> MNESVKEIPDVLKSQCGFNCLTDISHSSFNEFRQQVSEHLSWSETHDLYHDAQQAQKDNRLYEARILKRANPQLQNAVHLAILAPNAELIGYNNQFSGRASQYVAPGTVSSMFSPAAYLTELYREARNLHASDSVYYLDTRRPDLKSMALSQQNMDIELSTLSLSNELLLESIKTESKLENYTKVMEMLSTFRPSGATPYHDAYENVREVIQLQDPGLEQLNASPAIAGLMHQASLLGINASISPELFNILTEEITEGNAEELYKKNFGNIEPASLAMPEYLKRYYNLSDEELSQFIGKASNFGQQEYSNNQLITPVVNSSDGTVKVYRITREYTTNAYQMDVELFPFGGENYRLDYKFKNFYNASYLSIKLNDKRELVRTEGAPQVNIEYSANITLNTADISQPFEIGLTRVLPSGSWAYAAAKFTVEEYNQYSFLLKLNKAIRLSRATELSPTILEGIVRSVNLQLDINTDVLGKVFLTKYYMQRYAIHAETALILCNAPISQRSYDNQPSQFDRLFNTPLLN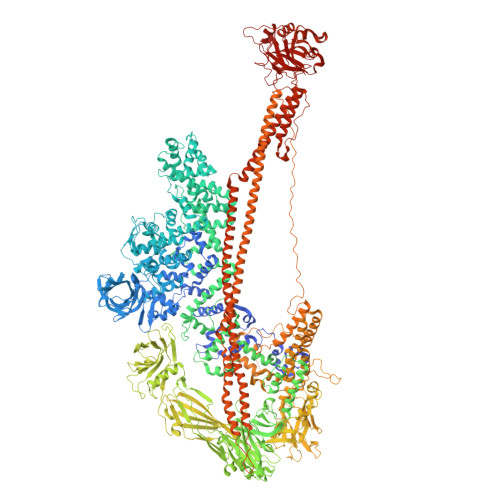GQYFSTGDEEIDLNSGSTGDWRKTILKRAFNIDDVSLFRLLKITDHDNKDGKIKNNLKNLSNLYIGKLLADIHQLTIDELDLLLIAVGEGKTNLSAISDKQLATLIRKLNTITSWLHTQKWSVFQLFIMTSTSYNKTLTPEIKNLLDTVYHGLQGFDKDKADLLHVMAPYIAATLQLSSENVAHSVLLWADKLQPGDGAMTAEKFWDWLNTKYTPGSSEAVETQEHIVQYCQALAQLEMVYHSTGINENAFRLFVTKPEMFGAATGAAPAHDALSLIMLTRFADWVNALGEKASSVLAAFEANSLTAEQLADAMNLDANLLLQASIQAQNHQHLPPVTPENAFSCWTSINTILQWVNVAQQLNVAPQGVSALVGLDYIQSMKETPTYAQWENAAGVLTAGLNSQQANTLHAFLDESRSAALSTYYIRQVAKAAAAIKSRDDLYQYLLIDNQVSAAIKTTRIAEAIASIQLYVNRALENVEENANSGVISRQFFIDWDKYNKRYSTWAGVSQLVYYPENYIDPTMRIGQTKMMDALLQSVSQSQLNADTVEDAFMSYLTSFEQVANLKVISAYHDNINNDQGLTYFIGLSETDAGEYYWRSVDHSKFNDGKFAANAWSEWHKIDCPINPYKSTIRPVIYKSRLYLLWLEQKEITKQTGNSKDGYQTETDYRYELKLAHIRYDGTWNTPITFDVNKKISELKLEKNRAPGLYCAGYQGEDTLLVMFYNQQDTLDSYKNASMQGLYIFADMASKDMTPEQSNVYRDNSYQQFDTNNVRRVNNRYAEDYEIPSSVSSRKDYGWGDYYLSMVYNGDIPTINYKAASSDLKIYISPKLRIIHNGYEGQKRNQCNLMNKYGKLGDKFIVYTSLGVNPNNSSNKLMFYPVYQYSGNTSGLNQGRLLFHRDTTYPSKVEAWIPGAKRSLTNQNAAIGDDYATDSLNKPDDLKQYIFMTDSKGTATDVSGPVEINTAISPAKVQIIVKAGGKEQTFTADKDVSIQPSPSFDEMNYQFNALEIDGSGLNFINNSASIDVTFTAFAEDGRKLGYESFSIPVTLKVSTDNALTLHHNENGAQYMQWQSYRTRLNTLFARQLVARATTGIDTILSMETQNIQEPQLGKGFYATFVIPPYNLSTHGDERWFKLYIKHVVDNNSHIIYSGQLTDTNINITLFIPLDDVPLNQDYHAKVYMTFKKSPSDGTWWGPHFVRDDKGIVTINPKSILTHFESVNVLNNISSEPMDFSGANSLYFWELFYYTPMLVAQRLLHEQNFDEANRWLKYVWSPSGYIVHGQIQNYQWNVRPLLEDTSWNSDPLDSVDPDAVAQHDPMHYKVSTFMRTLDLLIARGDHAYRQLERDTLNEAKMWYMQALHLLGDKPYLPLSTTWSDPRLDRAADITTQNAHDSAIVALRQNIPTPAPLSLRSANTLTDLFLPQINEVMMNYWQTLAQRVYNLRHNLSIDGQPLYLPIYATPADPKALLSAAVATSQGGGKLPESFMSLWRFPHMLENARGMVSQLTQFGSTLQNIIERQDAEALNALLQNQAAELILTNLSIQDKTIEELDAEKTVLEKSKAGAQSRFDSYGKLYDENINAGENQAMTLRASAAGLTTAVQASRLAGAAADLVPNIFGFAGGGSRWGAIAEATGYVMEFSANVMNTEADKISQSETYRRRRQEWEIQRNNAEAELKQIDAQLKSLAVRREAAVLQKTSLKTQQEQTQSQLAFLQRKFSNQALYNWLRGRLAAIYFQFYDLAVARCLMAEQAYRWELNDDSARFIKPGAWQGTYAGLLAGETLMLSLAQMEDAHLKRDKRALEVERTVSLAEVYAGLPKDNGPFSLAQEIDKLVSQGSGSAGSGNNNLAFGAGTDTKTSLQASVSFADLKIREDYPASLGKIRRIKQISVTLPALLGPYQDVQAILSYGDKAGLANGCEALAVSHGMNDSGQFQLDFNDGKFLPFEGIAIDQGTLTLSFPNASMPEKGKQATMLKTLNDIILHIRYTIK> MVDATRVPMDERFRTLKKKLEEGMVFTEYEQIP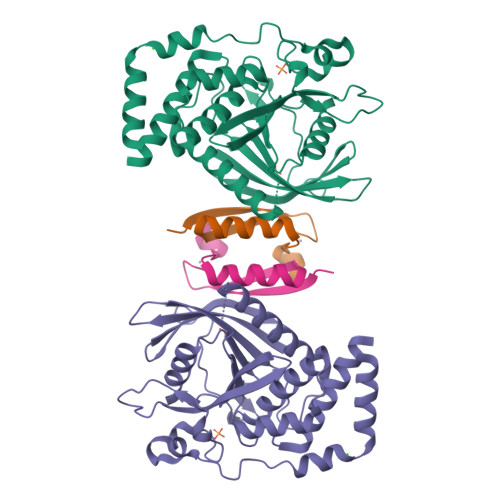KKKANGIFSTAALPENAERSRIREVVPYEENRVELIPTKENNTGYINASHIKVVVGGAEWHYIATQGPLPHTCHDFWQMVWEQGVNVIAMVTAEEEGGRTKSHRYWPKLGSKHSSATYGKFKVTTKFRTDSVCYATTGLKVKHLLSGQERTVWHLQYTDWPDHGCPEDVQGFLSYLEEIQSVRRHTNSMLEGTKNRHPPIVVHCSAGVGRTGVLILSELMIYCLEHNEKVEVPMMLRLLREQRMFMIQTIAQYKFVYQVLIQFLQNSRLI;> GHMAEPQRHTMLCMCCKCEARIELVVESSADDLRAFQQLFLNTLSFVCPWCASQQ> VDPRAKWQPQDNDIQACDYWRHCSIAGNICDCSAGSLTSCPPGTLVASGSWVGSCYNPPDPNKYITAYRDCCGYNVSGRCACLNTEGELPVYNKD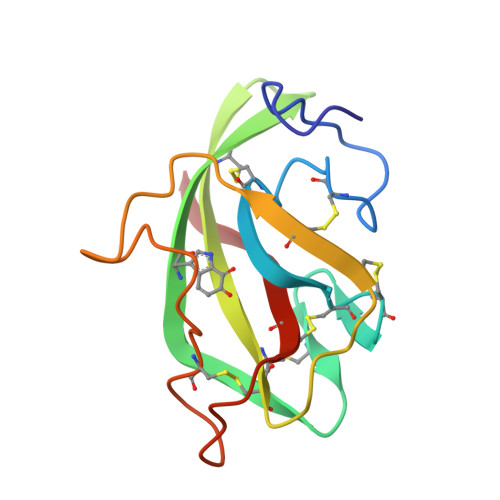ANDIIWCFGGEDGMTYHCSISPVSGA> SPREQDSESQTLDKVYQMKSKPRGYCLIINNHNFAKAREKVPKLHSIRDRNGTHLDAGALTTTFEELHFEIKPHDDCTVEQIYEILKIYQLMDHSN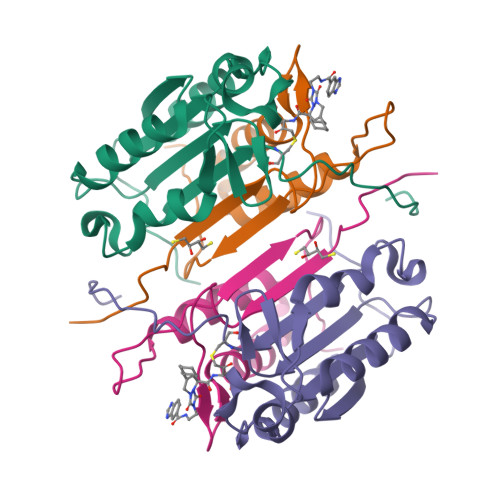MDCFICCILSHGDKGIIYGTDGQEAPIYELTSQFTGLKCPSLAGKPKVFFIQACQGDNYQKGIPVETD;> LSSPQTRYIPDEADFLLGMATVNNCVSYRNPAEGTWYIQSLCQSLRERCPRGDDILTILTEVNYEVSNKDDKKNMGKQMPQPTFTLRKKLVFPSD> MGHHHHHHMTTDDLLTRYRANPAMMKNLKLSDIRGALLKFAKDQVGSRFIQQELASSKDRFEKDSIFDEVVSNADELVDDIFGNYVVQKFFEYGEERHWARLVDAIIDRVPEYAFQMYACRVLQKALEKINEPLQIKILSQIRHVIHRCMKDQNGCRVVQKAIEKVSPQYVQFIVDTLLESSNTIYEMSVDPYGCRVVQRCLEHCSPSQTKPVIGQIHKRFDEIANNQYGNYVVQHVIEHGSEEDRMVIVTRVSNNLFEFATHKYSSNVIEKCLEQGAVYHKSMIVGAACHHQEGSVPIVV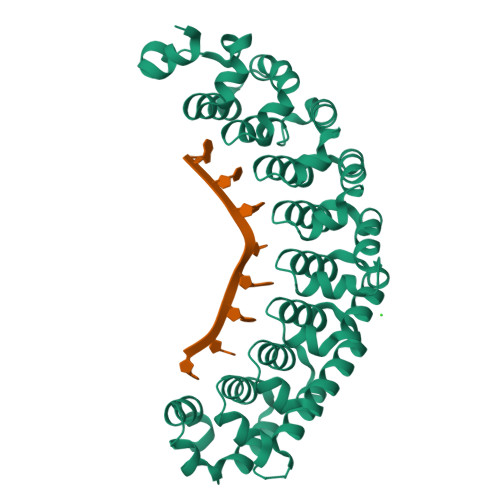QMMKDQYANYVVQKMFDQVTSEQRRELILTVRPHIPVLRQFPHGKHILAKLEKYFQKPA> MTKKGATKILFIYKLSKLNVYNNESYKIKLLFNHLYCIDNYNSIYFNLNGILIWLNVLHINI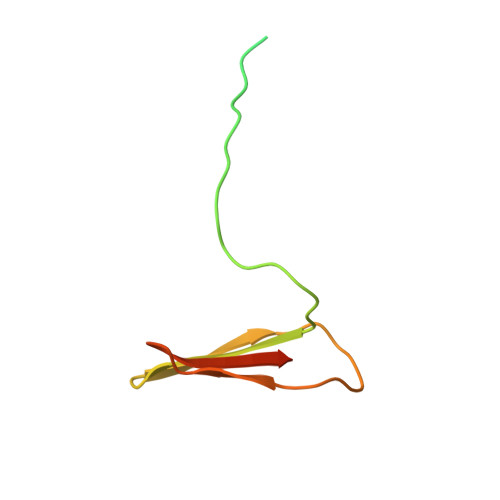ILIKYAFLILLNNLEYLIIFKYNIISIK>GFKQDIATIRGDLRTYAQDIFLAFLNKYPDERRYFKNYVGKSDQELKSMAKFGDHTEKVFNL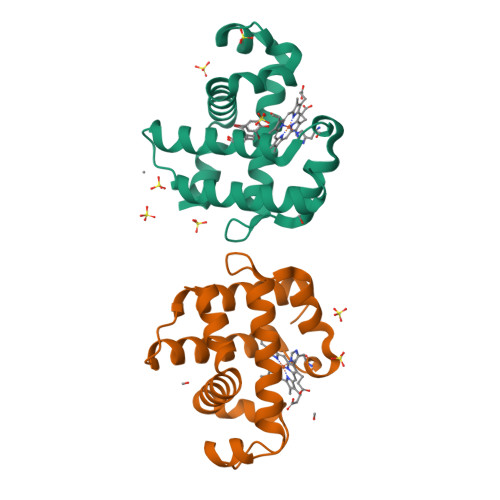MMEVADRATDCVPLASDANTLVQMKQHSSLTTGNFEKLFVALVEYMRASGQSFDSQSWDRFGKNLVSALSSAGMK[2x]>[2x]DCYCRIPACIAGERRYGT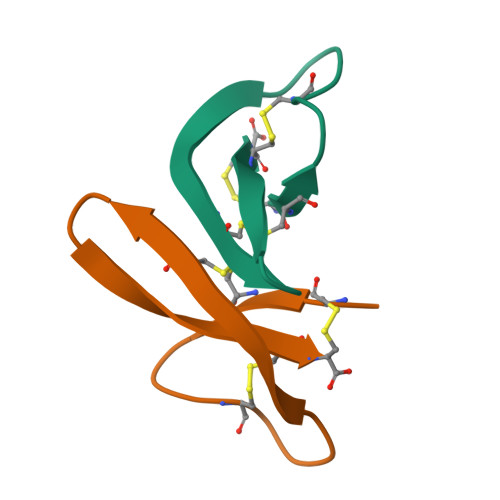CIYQGRLWAFCC>[2x]MFKDGSLIPYLTAGDPDKQSTLNFLLALDEYAGAIELGI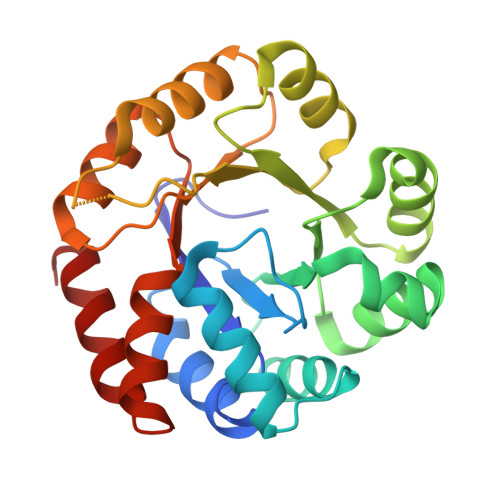PFSDPIADGKTIQESHYRALKNGFKLREAFWIVKEFRRHSSTPIVLMTYYNPIYRAGVRNFLAEAKASGVDGILVVDLPVFHAKEFTEIAREEGIKTVFLAAPNTPDERLKVIDDMTTGFVYLVSLYGTTGAREEIPKTAYDLLRRAKRICRNKVAVGFGVSKREHVVSLLKEGANGVVVGSALVKIIGEKGREATEFLKKKVEALLGI> MKKD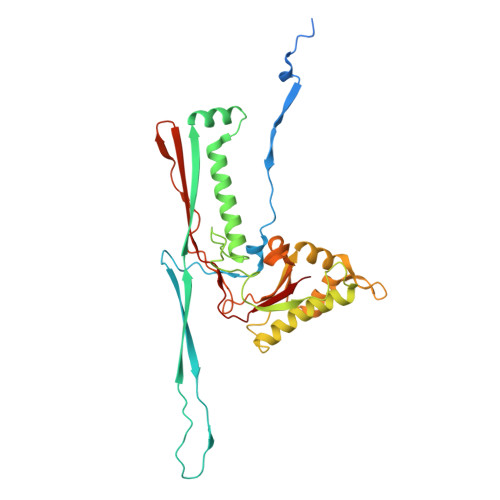LKFIKSVYDLKSFSDKAAFAKKTFKDEGGIILARNLEHVSSEIFTQEFAGLTFLQGGIVVNNEGGYATSVTKLKLKAEGGFRESGNDTNTTGKITLSGESDSIPVFTLEGESDWSEIELKQAELQNVNLPSRYFEAHAELYNRKIDELGYLGQTRTDGTQKTLGLLNYGFVASGAGDTAANLSGDNLYQAIADLITDQWAGVFNVETYKADRVVMPDTVYNICAKKILNSNGSEMSVLRALMTNFPTVTFGLTTKARDVGGTSRTTAYSSNRRAMQMRIPTPLNVSSVDQRGFKYYVESYFGVAGLDVIEDTAGRHLTGL>MLFGRLTERAQRVLAHAQEEAIRLNHSNIGTEHLLLGLMKEPEGIAAKVLESFNITEDKVIEEVEKLIGHGQDHVGTLHYTPRAKKVIELSMDEARKLHHNFVGTEHILLGLIRENEGVAARVFANLDLNITKARAQVVKALGNPEMSNKNAQASKSNNTPTLDSLARDLTVIAKDGTLDPVIGRDKEITRVIEVLSRRTKNNPVLIGEPGVGKTAIAEGLAQAIVNNEVPETLKDKRVMSLDMGTVVAGTKYRGEFEERLKKVMEEIQQAGNVILFIDELHTLVGAGGAEGAIDASNILKPALARGELQCIGATTLDEYRKNIEKDAALERRFQPVQVDEPSVVDTVAILKGLRDRYEAHHRINISDEAIEAAVKLSNRYVSDRFLPDKAIDLIDEASSKVRLKSHTTPNNLKEIEQEIEKVKNEKDAAVHAQEFENAANLRDKQTKLEKQYEEAKNEWKNAQNGMSTSLSEEDIAEVIAGWTGIPLTKINETESEKLLSLEDTLHERVIGQKDAVNSISKAVRRARAGLKDPKRPIGSFIFLGPTGVGKTELARALAESMFGDDDAMIRVDMSEFMEKHAVSRLVGAPPGYVGHDDGGQLTEKVRRKPYSVILFDEIEKAHPDVFNILLQVLDDGHLTDTKGRTVDFRNTIIIMTSNVGAQELQDQRFAGFGGSSDGQDYETIRKTMLKELKNSFRPEFLNRVDDIIVFHKLTKEELKEIVTMMVNKLTNRLSEQNINIIVTDKAKDKIAEEGYDPEYGARPLIRAIQKTIEDNLSELILDGNQIEGKKVTVDHDGKEFKYDIAEQTSETKTPSQA[10x]

The bacterial AAA+ chaperone ClpC associates with the peptidase ClpP to form a central proteolytic machinery of Gram-positive bacteria. The ClpC-ClpP machinery acts in regulatory and general proteolysis, controlling multiple cellular pathways and differentiation processes and is crucial for bacterial stress resistance and virulence. ClpC activity crucially relies on cooperation with adaptor proteins including MecA, that target specific substrates while concurrently stimulating ClpC ATPase activity. Here, we report on an unexpected mode of AAA+ chaperone control involving transition between an inactive resting state and a functional hexamer as revealed by determining the cryoEM-structures of S. aureus ClpC in absence and presence of MecA.

The structure of ClpC on its own was solved at 8.4 Å resolution using ~90.000 collected particles. Attempts of 3D classification and refinement using the existing ClpC-MecA structures failed to give a refined map, indicating that on its own, ClpC assumes a substantially different conformation. Indeed, reconstructions revealed that ClpC without MecA assembles into an oligomeric assembly made of two open spirals that interact via head-to-head contacts mainly mediated by the MDs (Figure 3A/B). The AAA+ domains are staggered with a rise of ~20 Å per subunit. N-domains domains are packed between MDs and are displaced so that they lie on top of the adjacent small AAA1 subdomain (Figure 3B/C). The MDs coiled-coils constitute the backbone of the spiral and mediate the spiral head-to-head contacts, which involve residues F436, R443 and D444 providing a structural rationale for the activated states of respective MD mutants. The MD-MD head-to-head interaction stops the formation of virtually infinite spirals as in the Hsp104 crystal arrangements allowing the formation of a compact, repressed ClpC reservoir. ATP addition caused formation of larger ClpC assemblies that eluted prior to ClpB hexamers and a 670 kDa standard protein, suggesting formation of ClpC complexes larger than hexamers. This was confirmed by static light scattering (SLS) measurements, revealing a molecular mass of ≈ 956 kDa corresponding to a decameric complex, consistent with cryoEM analysis. We define this large ClpC assembly as inactive resting state, as it strongly restricts binding of substrates, ClpP and adaptor proteins and does not allow for efficient ATP hydrolysis. As MecA-binding sites in N- and M-domains are not accessible in the resting state, we suggest that ClpC subunit dissociation is prerequisite for MecA binding.>NVYHDGACPEVKPVDNFDWSNYHGKWWEVAKYPNSVEKYGKCGWAEYTPEGKSVKVSNYHVIHGKEYFIEGTAYPVGDSKIGKIYHKLTYGGVTKENVFNVLSTDNKNYIIGYYCKYDEDKKGHQDFVWVL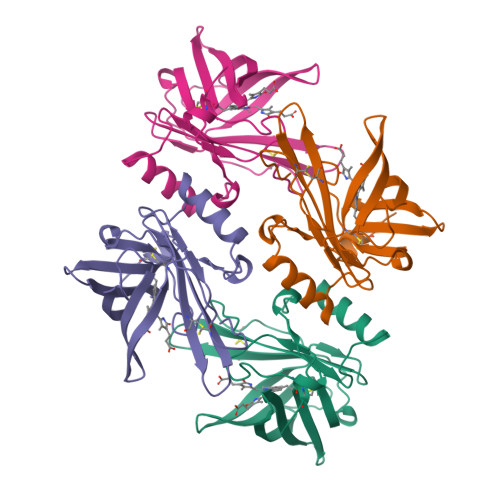SRSKVLTGEAKTAVENYLIGSPVVDSQKLVYSDFSEAACKVN[4x]> MAHHHHHHMKALAKLERGPGLTLTRVKKPEVGHNDVLIKIRRTAICGTDIHIWKWDDWAQKTIPVPMHVGHEYVGEIVEMGQEVRGFSIGDRVSGEGHITCGFCRNCRAGRRHLC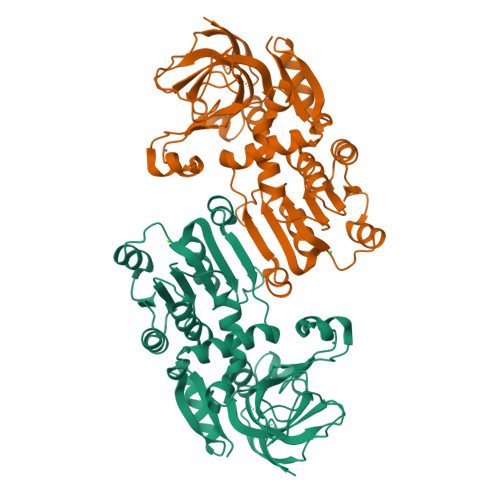RNTVGVGVNREGAFAEYLAIPAFNAFKIPPEISDDLAAIFDPFGNATHTALSFNLVGEDVLITGAGPIGVMAVAIAKHVGARNVVITDINDYRLDLARRMGATRAVNVSRESLRDVMADLHMTEGFDVGLEMSGVPSAFTSLLESMNHGGKVALLGIPPAQTAIDWNQVIFKGLEIKGIYGREMFETWYKMVAMLQSGLDLSPIITHRFAVDDYEKGFAAMLSGESGKVILDWAAA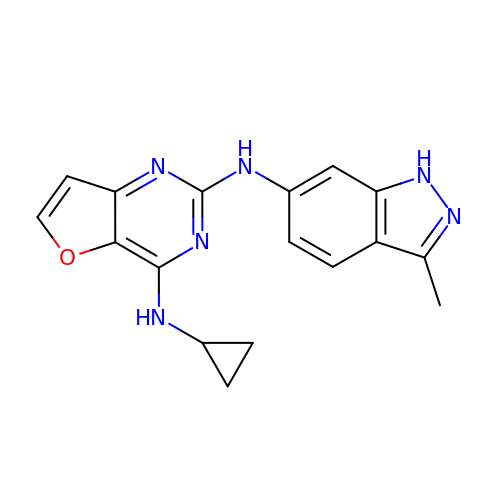N~4~-cyclopropyl-N~2~-(3-methyl-1H-indazol-6-yl)furo[3,2-d]pyrimidine-2,4-diamine | C17 H16 N6 O | MDWXVGCLSBQVMP-UHFFFAOYSA-N>MDKR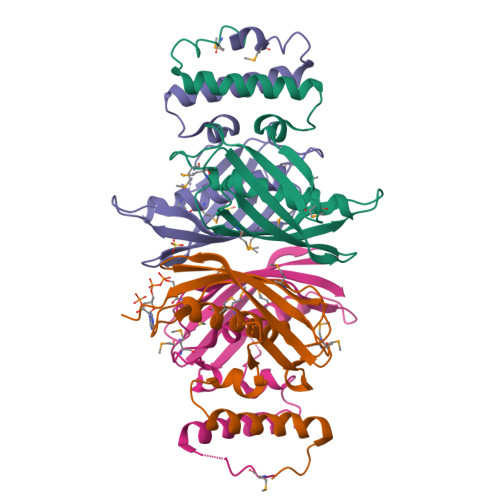LQQDRIVDKMERFLSTANEEEKDVLSSIVDGLLAKQERRYATYLASLTQIESQEREDGRFEVRLPIGPLVNNPLNMVHGGITATLLDTAMGQMVNRQLPDGQSAVTSELNIHYVKPGMGTYLRAVASIVHQGKQRIVVEGKVYTDQGETVAMGTGSFFVLRSRGLEHHHHHH[4x]>[2x]DDPPATVYRYDSRPPEDVFQNGFTAWGNNDNVLEHLTGRSCQVGSSNSAFVSTSSSRRYTEVYLEHRMQEAVEAERAGRGTGHFIGYIYEVRADNNFYGAASSYFEYVDTY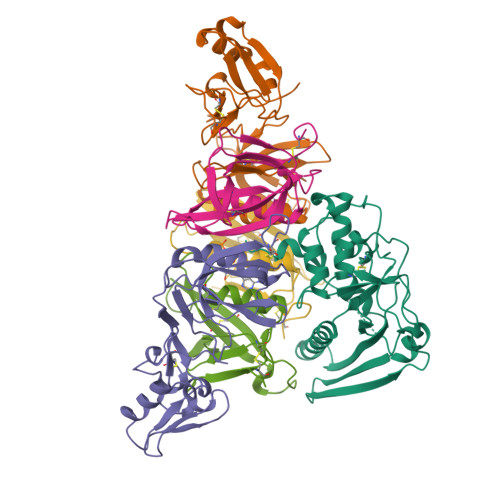GDNAGRILAGALATYQSEYLAHRRIPPENIRRVTRVYHNGITGETTTTEYSNARYVSQQTRANPNPYTSRRSVASIVGTLVRMAPVVGACMARQAESSEAMAAWSERAGEAMVLVYYESIAYSF;>STPGIVIPPQEQITQHGSPYGRCANKTRALTVAELRGSGDLQEYLRHVTRGWSIFALYDGTYLGGEYGGVIKDGTPGGAFDLKTTFCIMTTRNTGQPATDHYYSNVTATRLLSSTNSRLCAVFVRSGQPVIGACTSPYDGKYWSMYSRLRKMLYLIYVAGISVRVHVSKEEQYYDYEDATFETYALTGISICNPGSSLC[2x];>[2x]VAPGIVIPPKALFTQQGGAYGRCPNGTRALTVAELRGNAELQTYLRQITPGWSIYGLYDGTYLGQAYGGIIKDAPPGAGFIYRETFCITTIYKTGQPAADHYYSKVTATRLLASTNSRLCAVFVRDGQSVIGACASPYEGRYRDMYDALRRLLYMIYMSGLAVRVHVSKEEQYYDYEDATFQTYALTGISLCNPAASIC;>[4x]DVPYVLVKTNMVVTSVAMKPYEVTPTRMLVCGIAAKLGAAASSPDAHVPFCFGKDLKRPGSSPMEVMLRAVFMQQRPLRMFLGPKQLTFEGKPALELIRMVECSGKQDCP;>GLPTHLYKNFTVQELALKLKGKNQEFCLTAFMSGRSLVRACLSDAGHEHDTWFDTMLGFAISAYALKSRIALTVEDSPYPGTPGDLLELQICPLNGYCE[2x]6-[3-(4,4-difluoropiperidin-1-yl)prop-1-yn-1-yl]-4-methylpyridin-2-amine | C14 H17 F2 N3 | 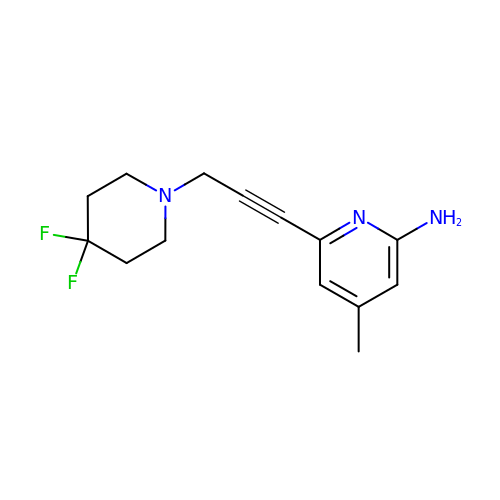SHKLMOHQZBDLIM-UHFFFAOYSA-N>[2x]ALGVVGVLESYIGSINNITKQSACVAMSKL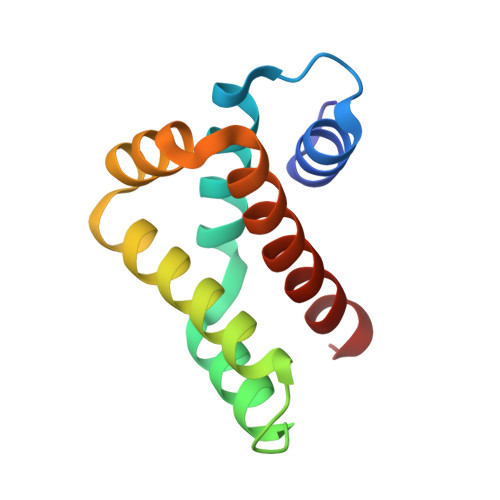LTELNSDDIKKLRDNEELNSPKIRVYNTVISYIESNRKNNKQTIHLLKRLPADVLKKTIKNTLDIHKSITINN> MADEKPK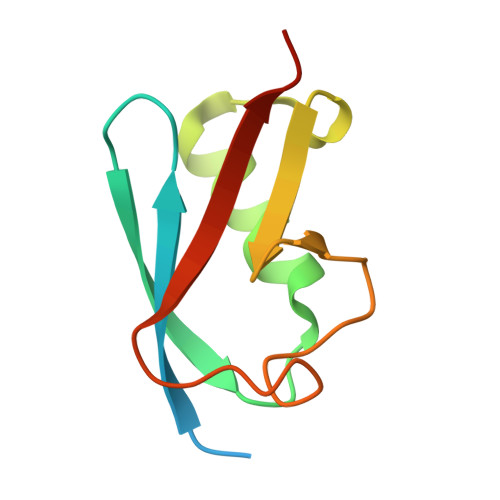EGVKTENNDHINLKVAGQDGSVVQFKIKRHTPLSKLMKAYCERQGLSMRQIRFRFDGQPINETDTPAQLEMEDEDTIDVFQQQTGG> MVMTDQAITFDDVLLVPSYNHHESRRVVETTSTDRLGKLTLNLPVISANMDTITESNMANFMHSKGAMGALHRFMTIEENIQEFKKCKGPVFVSVGCTENELQRAEALRDAGADFFCVDVAHAHAKYVGKTLKSLRQLLGSRCIMAGNVATYAGADYLASCGADIIKAGIGGGSVCSTRIKTGFGVPMLTCIQDCSRADRSIVADGGIKTSGDIVKALAFGADFVMIGGMLAGSAPTPGEVFQKDDGSKVKRYRGMASREAQEAFLGQMHEWKTAEGVATEVPFKENPDGIIADIIGGLRSGLTYAGADSISELQRKLNYV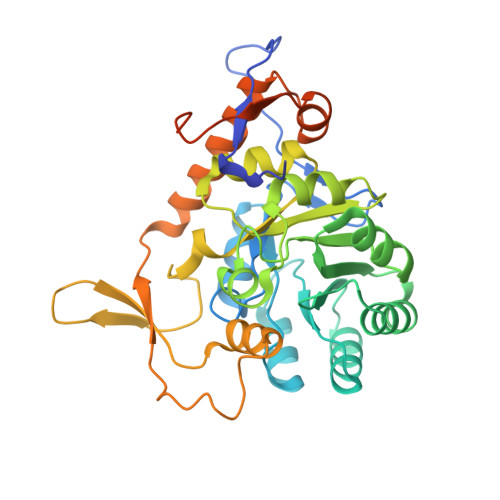IVTQAGRIESLPHKLLEGAENLYFQSHHHHHHWSHPQFEK> GSPGILAPLAPGSE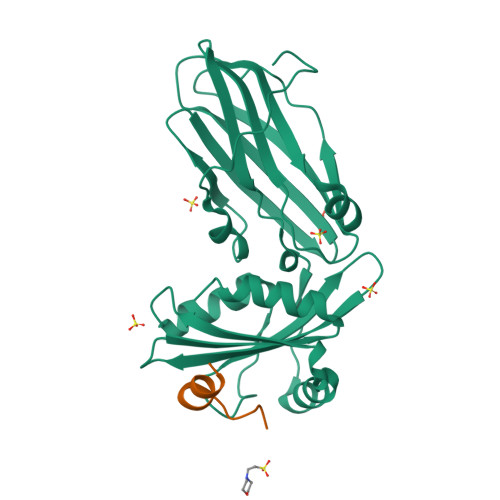DNFARFVCKNNGVLFENQLLQIGLKSEFRQNLGRMFIFYGNKTSTQFLNFTPTLICADDLQTNLNLQTKPVKPTVDGGAQVQQVVNIECISDFTEAPVLNIQFRYGGTFQNVSVKLPITLNKFFQPTEMASQDFFQRWKQLSNPQQEVQNIFKAKHPMDTEITKAKIIGFGSALLEEVDPNPANFVGAGIIHTKTTQIGCLLRLEPNLQAQMYRLTLRTSKDTVSQRLCELLSEQF;> QSEEQVSKNLFGPPLESAFDHED3,6-dimethyl-2~{H}-1,2,4-triazin-5-one | C5 H7 N3 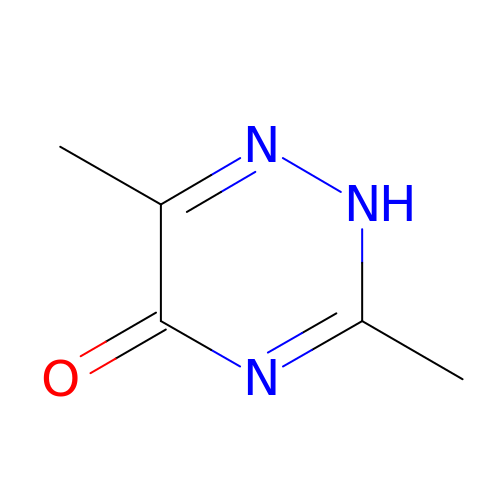O | WZMOVTWDPULYIG-UHFFFAOYSA-N> MTITPQNLIALLPLLIVGLTVVVVMLSIAWRRNHFLNATLSVIGLNAALVSLWFVGQAGAMDVTPLMRVDGFAMLYTGLVLLASLATCTFAYPWLEGY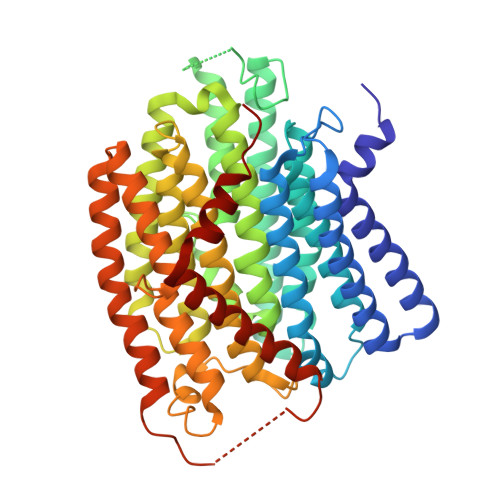NDNKDEFYLLVLIAALGGILLANANHLASLFLGIELISLPLFGLVGYAFRQKRSLEASIKYTILSAAASSFLLFGMALVYAQSGDLSFVALGKNLGDGMLNEPLLLAGFGLMIVGLGFKLSLVPFHLWTPDVYQGAPAPVSTFLATASKIAIFGVVMRLFLYAPVGDSEAIRVVLAIIAFASIIFGNLMALSQTNIKRLLGYSSISHLGYLLVALIALQTGEMSMEAVGVYLAGYLFSSLGAFGVVSLMSSPYRGPDADSLFSYRGLFWHRPILAAVMTVMMLSLAGIPMTLGFIGKFYVLAVGVQAHLWWLVGAVVVGSAIGLYYYLRVAVSLYLHAPEQPGRDAPSNWQYSAGGIVVLISALLVLVLGVWPQPLISIVRLAMPLM>MKTPTIPTLLGPDGMTSLREYAGYHGGGSGFGGQLRSWNPPSESVDAALLPNFTRGNARADDLVRNNGYAANAIQLHQDHIVGSFFRLSHRPSWRYLGIGEEEARAFSREVEAAWKEFAEDDCCCIDVERKRTFTMMIREGVAMHAFNGELFVQATWDTSSSRLFRTQFRMVSPKRISNPNNTGDSRNCRAGVQINDSGAALGYYVSEDGYPGWMPQKWTWIPRELPGGRASFIHVFEPVEDGQTRGANVFYSVMEQMKMLDTLQNTQLQSAIVKAMYAATIESELDTQSAMDFILGANSQEQRERLTGWIGEIAAYYAAAPVRLGGAKVPHLMPGDSLNLQTAQDTDNGYSVFEQSLLRYIAAGLGVSYEQLSRNYAQMSYSTARASANESWAYFMGRRKFVASRQASQMFLCWLEEAIVRRVVTLPSKARFSFQEARSAWGNCDWIGSGRMAIDGLKEVQEAVMLIEAGLSTYEKECAKRGDDYQEIFAQQVRETMERRAAGLKPPAWAAAAFESGLRQSTEEEKSDSRAA[12x];>MTRQEELAAARAALHDLMTGKRVATVQKDGRRVEFTATSVSDLKKYIAELEVQTGMTQRRRGPAGFYV[12x]

The temperate phage lambda, which infects the bacterium Escherichia coli, belongs to Siphoviridae. The virion of the lambda phage comprises an icosahedral head and a long flexible tail. The tail, which comprises the tail tube and tail tip, connects with the head through the neck. The neck–tail complex comprises a channel formed by stacked 12-fold and hexameric rings and a 3-fold symmetrical tip.

The adaptor ring, which is formed by 12 copies of gpW, is assembled below the portal. A total of 65 residues (4–68) of the 68-residue adaptor protein gpW were resolved. The structure of gpW comprises 3 domains: a β-hairpin (residues 23–36), a two-α-helix bundle (residues 4–22 and 37–54), and an extended C-arm (residues 55–68). The assembly of the adaptor relies on hydrophobic interactions among the subunits of gpW. The interactions of the adjacent gpW subunits are further reinforced by interactions between the adjacent β-hairpin domains, which form a β-barrel. Compared with the NMR structure of a gpW monomer in solution, the β-hairpin in our gpW structure undergoes a 90° rotation, from parallel to vertical with respect to the two-α-helix bundle domain, which facilitates the formation of the β-barrel structure. The assembly of the adaptor on the portal mainly relies on the electrostatic interactions between the electropositive adaptor top and the electronegative portal bottom. In addition, the C-arm, which is absent from the NMR structure, interacts with residues 320–324 of the portal wing through β-sheet augmentation.>SLTAPPKEAARPTLMPRAQSYKDLTHLPAPTGKIFVSVYNIQDETGQFKPYPASNFSTAVPQSATAMLVTALKDSRWFIPLERQGLQNLLNERKIIRAAQENGTVAINNRIPLQSLTAANIMVEGSIIGYESNVKSGGVGARYFGIGADTQYQLDQIAVNLRVVNVSTGEILSSVNTSKTILSYEVQAGVFRFIDYQRLLEGEVGYTSNEPVMLCLMSAIETGVIFLINDGIDRGLWDLQNKAERQNDILVK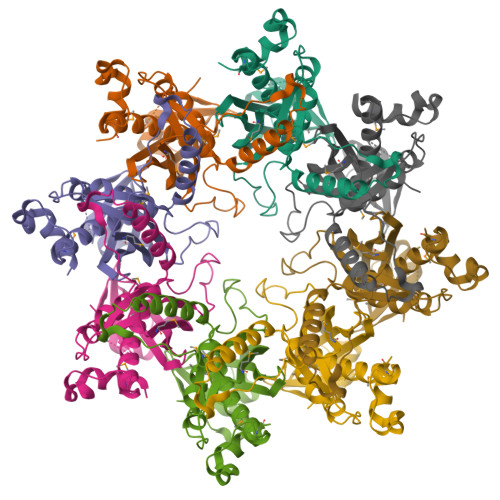YRHMSVPPES[16x]> MKEVARVRNLNRIIMGKYEIEPWYFSPYPIELTDED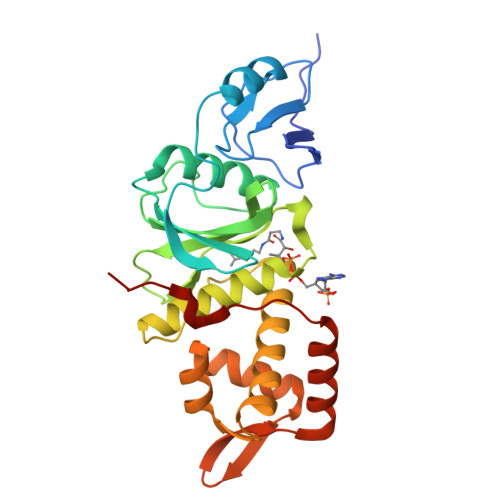FIYIDDFTLQYFGSKKQYERYRKKCTLRHPPGNEIYRDDYVSFFEIDGRKQRTWCRNLCLLSKLFLDHKTLYYDVDPFLFYCMTRRDELGHHLVGYFSKEKESADGYNVACILTLPQYQRMGYGKLLIEFSYELSKKENKVGSPQKPLSDLGLLSYRAYWSDTLITLLVEHQKEITIDEISSMTSMTTTDILHTAKTLNILRYYKGQHIIFLNEDILDRYNRLKAKKRRTIDPNRLIWKPPV>[10x]MLKTISPLISPELLKVLAEMGHGDEIIFSDAHFPAHSMGPQVIR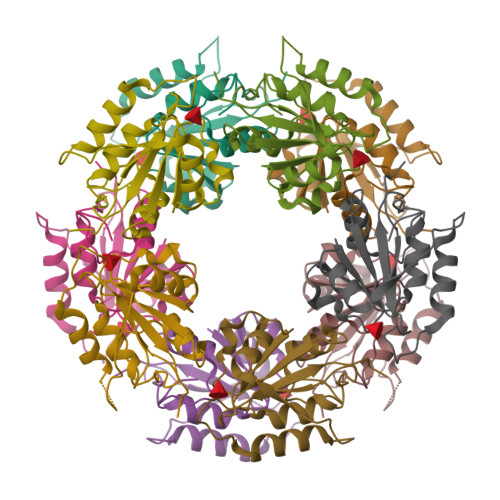ADGLLVSDLLQAIIPLFELDSYAPPLVMMAAVEGDTLDPEVERRYRNALSLQAPCPDIIRINRFAFYERAQKAFAIVITGERAKYGNILLKKGVTP>SGPWMCYPGQAFQVPALPACRPLLRLQCNGSQVPEAVLRDCCQQLAHISEWCRCGALYSMLDSMYKEHGAQEGQAGTGAFPRCRREVVKLTAA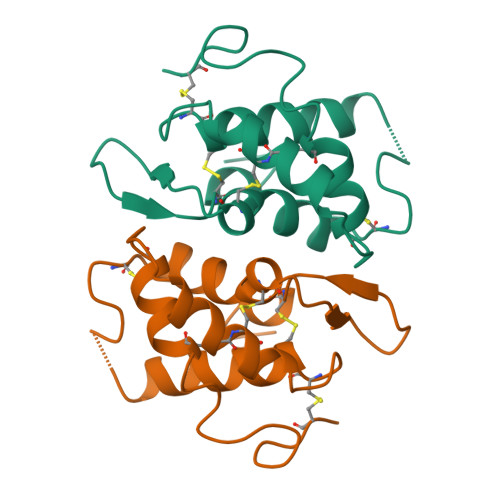SITAVCRLPIVVDASGDGAYVCKDVAAYPDA[4x]> MLRRTEIALKKGWTHNPGHTRRGGKNLAWRPKISDAKLSQFVPLALVHPRRHPNNWQERQFNALGYTK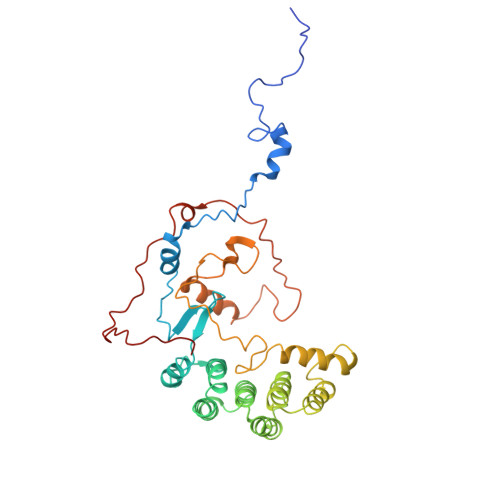WPKDIGFYNAGDNFEVTPEAAWRLYVHARDEPYWGKLHCEKTIITLLPVVEKAPKENMERVLDVFRHYLKRYGADHYIYNAVMQAAAFAKNYEQAEQLFKEMETLGLEPNAQSYVNMMLAAKLCGLPPEKSEAYFKRAVKDGAMQSVMRMDTEFRMWMDQLDRLGSFTASSGYLSVNEEGAKPMPRDMWAIWGWHRSESKFISRRDLIMQQVRARVHSGKELVGTVYTKTRRQPWAKFNGMLRHDYNGPSYRAPTIFPDAPEYTNEAGHKAF8-[4-[2-[4-[3,5-bis(chloranyl)phenyl]piperidin-1-yl]ethyl]pyrazol-1-yl]-3~{H}-pyrido[3,4-d]pyrimidin-4-one 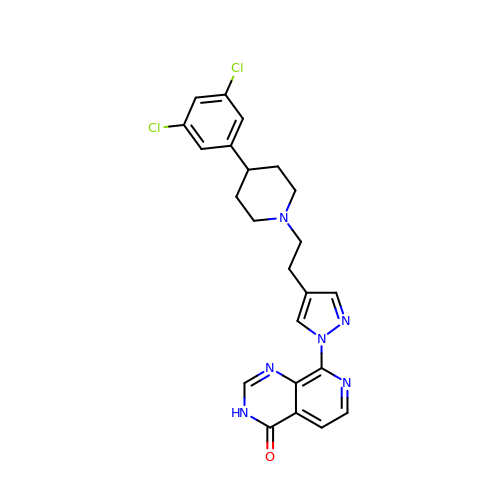| C23 H22 Cl2 N6 O | RLRGPZGIQMEBLC-UHFFFAOYSA-N> MKLAIAALLCASAAAFAPAPASKVSTALNVNELEIGATAPLGVYDPLGWLDGEPENFERRRAVERKHGRVAMAAVVGTIVHNNHITFDGYLSPSANLKFSDIPTGVDGIRAIPTAGLLQILFFFALVELAWMPASKYDGDYG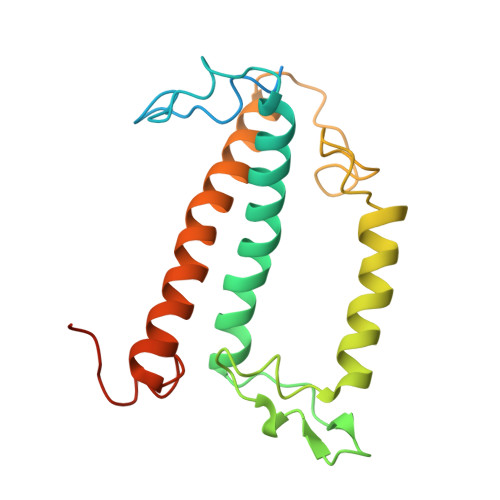VGWFGSNIEDPEEKARKLNVELNNGRAAMMGIMGNMVTECITGQTMYEQYAAGHFSPFGDGQGAF>MDDLLQRVRRCEALQQPEWGDPSRLRDVQAYLRGSPALIRAGDILALRATLARVARGEALVVQCGDCAEDMDDHHAENVARKAAVLELLAGALRLAGRRPVIRVGRIAGQYAKPRSKPHEQVGEQTLPVYRGDMVNGREAHAEQRRADPQRILKGYAAARNIMRHLGWDAASGQEANASPVWTSHEMLLLDYELSMLREDEQRRVYLGSTHWPWIGERTRQVDGAHVALLAEVLNPVACKVGPEIGRDQLLALCERLDPRREPGRLTLIARMGAQKVGERLPPLVEAVRAAGHPVIWLSDPMHGNTIVAPCGNKTRLVRSIAEEVAAFRLAVSGSGGVAAGLHLETTPDDVTECVADSSGLHQVSRHYTSLCDPRLNPWQALSAVMAWSGAEAIPSATFPLETVA[2x]

PhzC encodes a putative 3-deoxy-d-arabino-heptulosonate 7-phosphate (DAH7P) synthase (DAH7PS), which catalyses the aldol-like condensation reaction between phosphoenolpyruvate (PEP) and erythrose 4-phosphate (E4P) to form DAH7P as the first committed step of the shikimate pathway, en route to chorismate. Although less than 10% sequence identity exists between the type I and II DAH7PS groupings, all characterised examples of DAH7PSs share a common (β/α)8-barrel fold, a common divalent metal-ion binding site and conservation of almost all of the residues involved with E4P and PEP binding. In comparison, P. aeruginosa expresses two type Iα and two type II DAH7PSs. The type II DAH7PSs are encoded by the ORFs PA1901 (and duplicated as PA4212) and PA2843 (PaeDAH7PSPA1901 and PaeDAH7PSPA2843 respectively).

The crystal structure of PaeDAH7PSPA1901 (phzC) was solved (resolution 2.70 Å, Rfree = 0.280) in complex with the substrate PEP and a Co2+ ion, with attached water molecule, bound at the active site, revealing for the first time the structure of a short-form type II DAH7PS that is involved in secondary (here phenazine) metabolism. PaeDAH7PSPA1901 crystallised in the space group C2221, with two DAH7PS chains present in the asymmetric unit. As with all DAH7PS structures reported to date, PaeDAH7PSPA1901 features a core (β/α)8-barrel fold, with an N-terminal extension to the core catalytic domain consistent with its membership of the type II DAH7PS family. Residues 1–59 form an N-terminal extension to the barrel, providing additional helices α0a, α0b and α0c, with strong structural homology to the equivalent helices in other structurally characterised type II DAH7PSs, in particular PaeDAH7PSPA2843. Residues 167–181 form loop α2β3, which lacks the inserted helices α2a and α2b as observed in both MtuDAH7PS and PaeDAH7PSPA2843. The PEP phosphate group is co-ordinated by atoms Glu217_N, Arg218_NH1, Arg271_NE, Arg271_NH2 and Lys240_NZ whereas the carboxylate group of PEP is co-ordinated by atoms Arg106_NH1 and Lys240_NZ. Unexpectedly, despite the absence of the α2a and α2b helices in PaeDAH7PSPA1901, which are associated with the formation of the minor interface in either PaeDAH7PSPA2843 or MtuDAH7PS, an alternative interaction to deliver a homotetrameric species is observed in PaeDAH7PSPA1901. This alternative minor interface for PaeDAH7PSPA1901 is formed through interaction between chains A and D (or chains B and C) by residues located primarily on loop α3β4 and is distinctive from the minor interface observed for all characterised DAH7PSs (both type I and II). For PaeDAH7PSPA1901, the alternative oligomeric interfaces and subsequent formation of a significantly different quaternary assembly, relative to either PaeDAH7PSPA2843 or MtuDAH7PS, disrupts completely the formation of any aromatic amino acid allosteric binding sites that are comparable with those observed for either PaeDAH7PSPA2843 or MtuDAHPS.2-heptylquinoline-3,4-diol | C16 H21 N O2 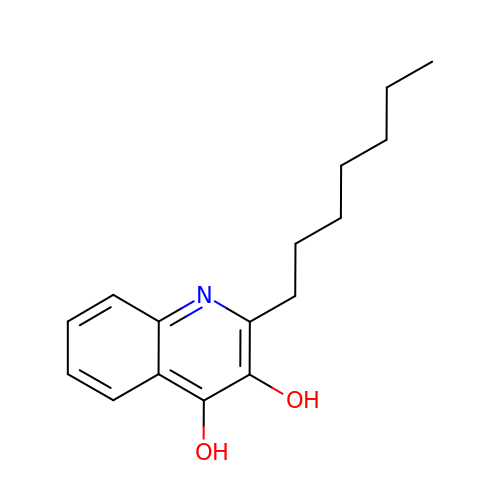| CEIUIHOQDSVZJQ-UHFFFAOYSA-N> EDLSPPSPP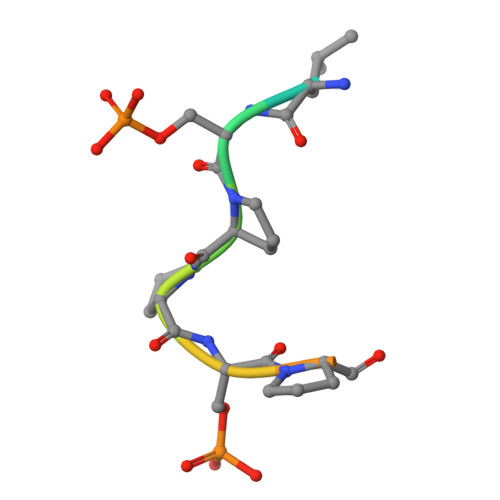LPK>[2x]MSLDKWEMERTDITMKHKLGGGQFGEVYEGVWKKYS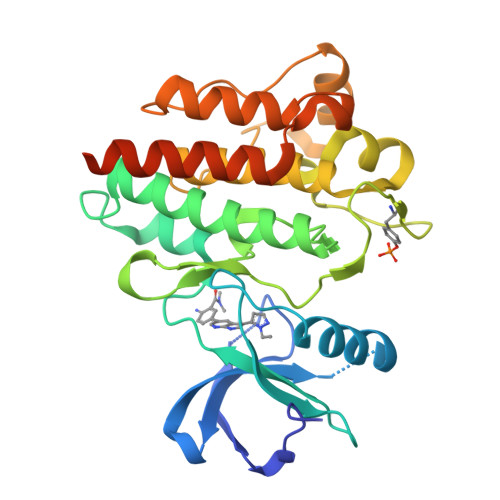LTVAVKTLKEDTMEVEEFLKEAAVMKEIKHPNLVQLLGVCTREPPFYIITEFMTYGNLLDYLRECNRQEVSAVVLLYMATQISSAMEYLEKKNFIHRDLAARNCLVGENHLVKVADFGLSRLMTGDTYTAHAGAKFPIKWTAPESLAYNKFSIKSDVWAFGVLLWEIATYGMSPYPGIDPSQVYELLEKDYRMERPEGCPEKVYELMRACWQWNPSDRPSFAEIHQAFETMFQESSISDEVEKELGKRGEGHHHHHH> MGGSHHHHHHENLYFQGMSQSNRELVVDFLSYKLSQKGYSWSQFSDVEENRTEAPEGTESEMETPSAINGNPSWHLADSPAVNGATGHSSS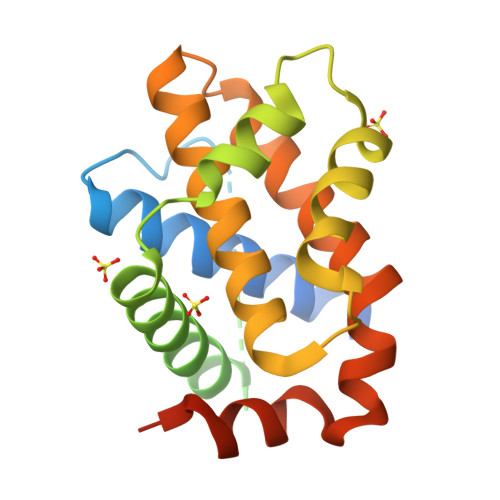LDAREVIPMAAVKQALREAGDEFELRYRRAFSDLTSQLHITPGTAYQSFEQVVNELFRDGVNWGRIVAFFSFGGALCVESVDKEMQVLVSRIAAWMATYLNDHLEPWIQENGGWDTFVELYGNNAAAESRKGQERFN>QSITDYNYKKPLHNDYQILDKSKIFGSNSGSFVMYSMAADAYYIYNEKESRKRYSPNSTYKIYLAMFGLDRHIINDENSRMSWNHKHYPFDAWNKEQDLNTAMQNSVNWYFERISDQIPKNYTATQLKQLNYGNKNLGSYKSYWMEDSLKISNLEQVIVFKNMMEQNNHFSKKAKNQLSSSLLIKKNEKYELYGKTGTGIVNGKYNNGWFVGYVITNHDKYYFATHLSDGKPSGKNAELISEKILK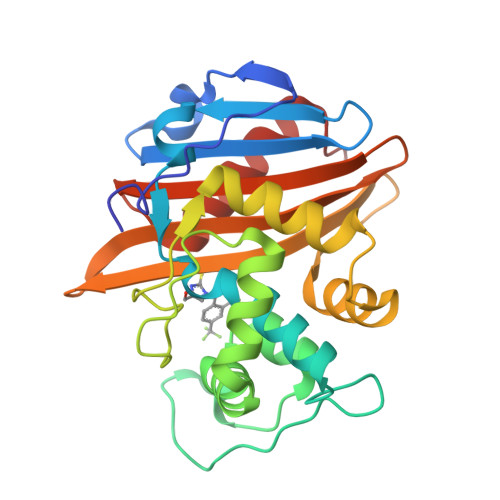EMGVLNGQ[2x]> FQPEFVESISNVSVAVGRDATFTCHVRHLGGYRVGWLKADTKAIQAIHENVITHNPRVTVSHLDQNTWNLHIKAVSEEDRGGYMCQLNTDPMKSQIGFLDVVIPPDFISEDTSSDVIVPEGSSVRLTCRARGYPEPIVTWRREDGNEIVLKDNVGTKTLAPSFRGEVLKLSKISRNEMGSYLCIASNGVPPSVSKRISLSIHFHPVIQVPNQLVGAPLGTDVQIECHVEASPKSINYWIKDTGEMIVTSGKYHVQESSQSMYETKMSMIVRKFQKDDVGSYRCIAKNSLGEVDSSIRLYEIPHHH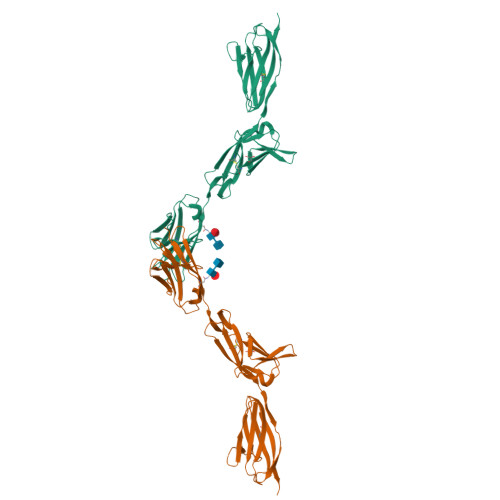HHH>[3x]GGSVLAERAGIDPTAILRDFDRGRTSTLPDGRTLREWDIVAVDKDFEIAPGIIFKGWSYNGRIPGPTLWAREGDALRIHFTNAGAHPHTIHFHGVHRATMDGTPGIGAGSIAPGQSFTYEFDATPFGTHLYHCHQSPLAPHIAKGLYGGFIVEPKEGRPPADDEMVMVMNGYNTDGGDDNEFYSVNGLPFHFMDFPVKVKQHELVRIHLINVLEYDPINSFHIHGNFFHYYPTGTMLTPSEYTDTISQVQ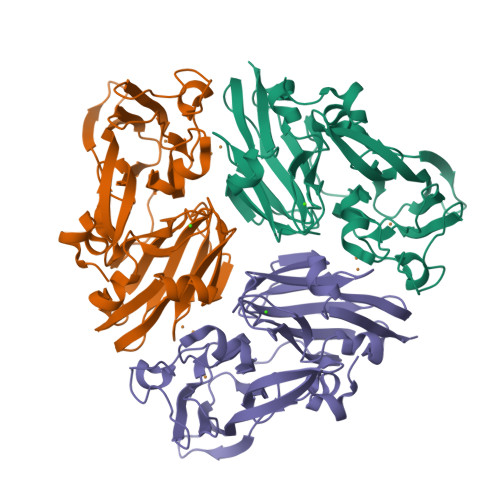GQRGILELRFPYPGKFMFHAHKTEFAELGWMGFFEVSA2-tert-butyl-1,3-dioxo-2,3-dihydro-1H-isoindole-5-carboxylic acid | C13 H13 N O4 | 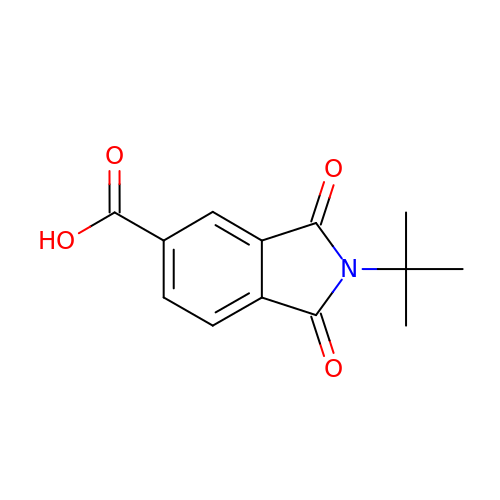XBMWXWYNYYVTMK-UHFFFAOYSA-N4-[(2S,4R)-1-acetyl-4-[(4-chlorophenyl)amino]-2-methyl-1,2,3,4-tetrahydroquinolin-6-yl]benzoic 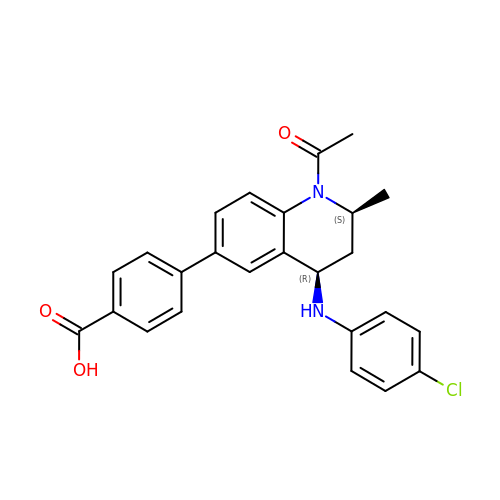acid | C25 H23 Cl N2 O3 | FAWSUKOIROHXAP-NPMXOYFQSA-N> NDDKIVVCYYGTWATYRTGLGKFDVDDIDPFLCTHLVYAFIGINAEGTALALDPELDVERGNFKQFTSLKEKNPNLKTLVAVGGWSEGSAQYSIMAAEPEYRQNFIQTSLAMILEYNFDGLDVDWEYPNRRDTVHGEDDIEQFSTLLKELREEFDNYGLLLTVAVSAVEEAAVQSYDVPSVAKYVDYIGVMTYDMHGAWDSVTG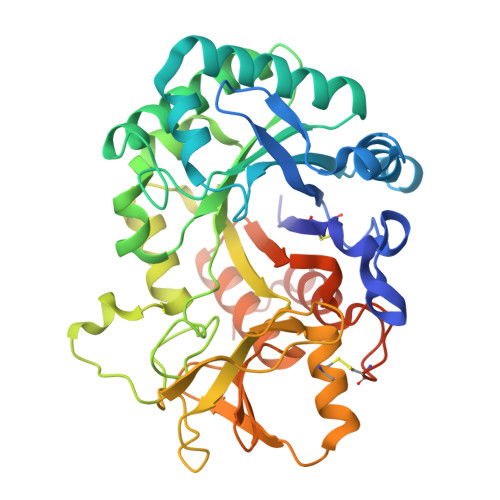HNAPLFISEGESAEQESTLYNVNNAVQYWLSAGCPPEKLVMGVPFYGRTFQLSDPSVNAPNSPSNGAGLAGPYTAESGYVGYNEFCYILQQESSWTVQTDNLAKVPYAFLDYNWVSFDNVESMTAKVEYANSFNLRGIMLWSIETDDFHGLCGEGTFPLLNTINTVLAEGSTEARHNNPPGHHHHHHHH ALISKIREN | C30 H53 N3 O6 | 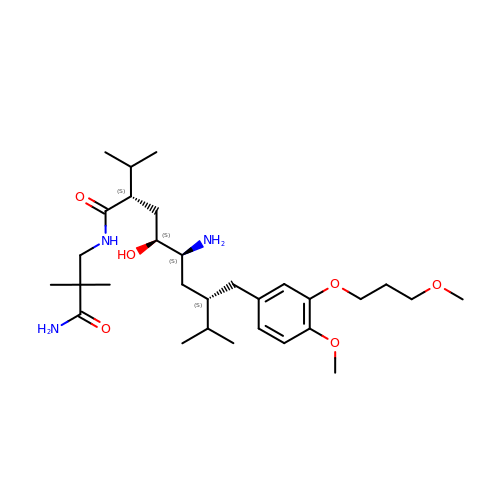UXOWGYHJODZGMF-QORCZRPOSA-N> MVIFDEHKFRTLFPEFADPAAYPDVRLQMYFDIACEFISDRDSPYRILNGKALEACLYLLTAHLLSLSTMQVQ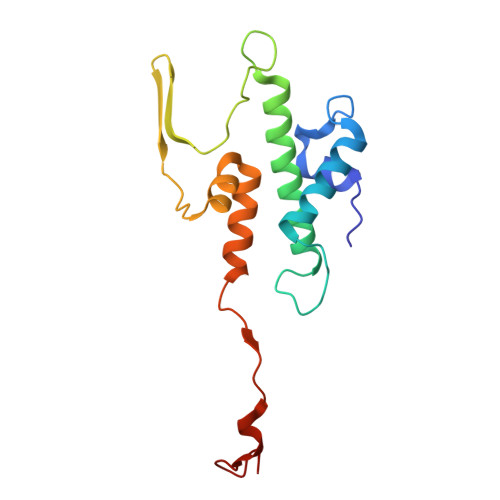GAAGGGVTAGGTQGGFITSATVGEVSVAKLAPPAKNGWQWWLSGTPYGQELWALLSVKAVGGFYIGGLPERRGFRKVGGTFW>[8x]SNAKEPSCMSSIIPGWFSEISPMWPGEAHSLKVEKILFQGKSDYQDVIVFQSATYGKVLVLDGVIQLTERDECAYQEMITHLPLCSISNPKKVLVIGGGDGGVLREVARHSSVEQIDICEIDKMVVDVAKQYFPNVAVGYEDPRVNLIIGDGVAFLKNAAEGTYDAVIVDSSDPIGPAKELFEKPFFESVNRALRPGGVVCTQAESLWLHMDIIEDIVSNCRDIFKGSVNYAWTSVPTYPSGVIGFMLCSSEGPQVDFKKPVSLIDTDESSIKSHCPLKYYNAEIHSAAFCLPSFAKKVIDSKAN

Longer polyamines are produced by aminopropyltransferases (APTs), enzymes that catalyze the transfer of an aminopropyl group from decarboxylated S-adenosylmethionine (dc-SAM), a universal cofactor of APTs, to a polyamine substrate. Thus, spermidine synthase (SPDS) utilizes PUT as the substrate for spermidine (SPD) biosynthesis. AtSPDS1 and AtSPDS2 share the fold of polyamine biosynthesis proteins with the characteristic two-domain topology. The active site of AtSPDS is formed between the N-terminal and C-terminal domains.

The structures of apo AtSPDS1 and AtSPDS2 present the PEG molecules (absorbed from the crystallization solution) bound within the active site. The conformation of this linear ligand mimics PUT, providing the information about the substrate binding mode inside the catalytic pocket. Additional β strand (Ser46-Ile48) is formed only in chain H of AtSPDS2 (one of the eight chains in the asymmetric unit) creating three-stranded β-sheet at the N-terminus. One subunit of the AtSPDS2 (chain H) presents the state, where no ligand is bound in the active site in neither the cofactor binding compartment nor in the polyamine groove. The conformation of this chain stands out from the others and presents the possible open conformation of the active site. Comparison of the chain H of AtSPDS2 in the open conformation with chain A of the AtSPDS1-CHA complex shows that the AtSPDS adopts two significantly different conformations. In the open conformation, the biggest conformational difference concerns the region with η6. The preceding loop uncoils and η6 is now moved toward α8, over 10 Å away from the position in the closed form. Therefore, the negatively charged active site is uncovered and ready to incorporate cofactor and substrate.>[6x]MEQTFIM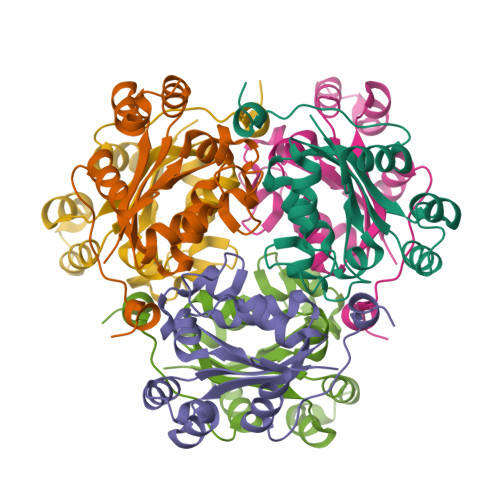IKPDGVQRGLIGEVICRFEKKGFTLKGLKLISVERSFAEKHYEDLSSKSFFSGLVDYIVSGPVVAMIWEGKNVVLTGRKIIGATNPAASEPGTIRGDFAIDIGRNVIHGSDSVESARKEIALWFPDGPVNWQSSVHPWVYET> SNATSSTEPDEVGGESFTIPVSSLRLRDPFILVDKKTSMYYLHFNNNLKIRVYKSKDLSTWKDEGYSFIAKSDFWGQQDFWAPDVYEYEGRYYLFTTFSNAGVKRGTSILVSDSPKGPFTPLVNKAITPSGWMCLDGSLYIDKEGNPWLLFCREWLETIDGEIYAQRLAKDLKTTEGDPYLLFKASEAPWVGSITS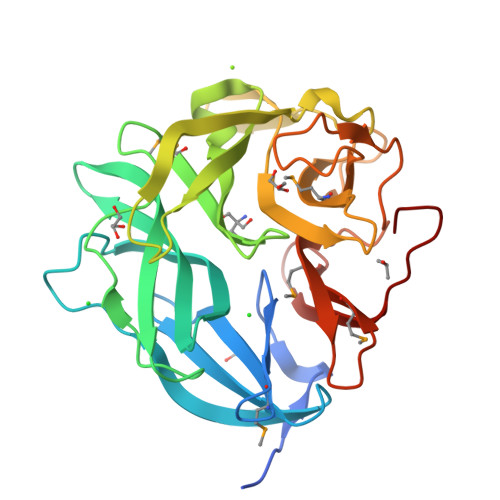SGVTGNVTDAPFIYRLDDGKLIMLWSSFRKTDGKYAIGQAVSASGNVLGPWVQEPETLNSDDGGHAMVFKDLKGRLMISYHAPNSQTEHPVITPIYIKDGKF>[2x]MIMSEMITRQQVTSGETIHVRTDPT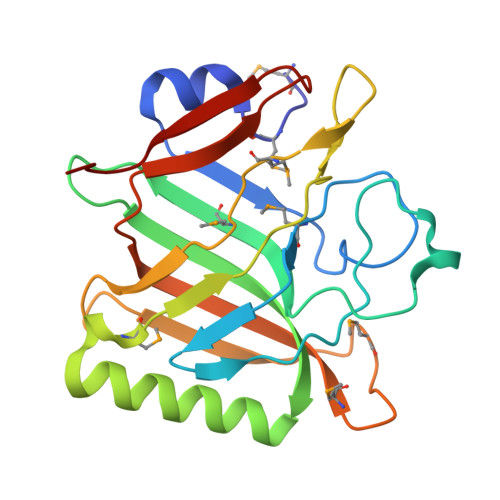ACIGSHPNCRMFIDSLTIAGEKLDKNIVAIDGGEDVTKADSATAAASVIRMSITPGSINPTISITLGVLIKSNVRTKIEEKVSSILQASATDMKIKLGNSNKKQEYKTDEAWGIMIDLSNLELYPISAKAFSISIEPTELMGVSKDGMRYHIISIDGLTTSQGSLPVCCAASTDKGVAKIGYIAAA> GPAFEFAVAMMKRN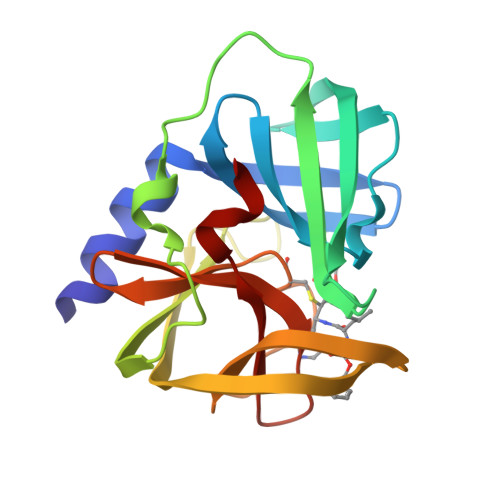SSTVKTEYGEFTMLGIYDRWAVLPRHAKPGPTILMNDQEVGVLDAKELVDKDGTNLELTLLKLNRNEKFRDIRGFLAKEEVEVNEAVLAINTSKFPNMYIPVGQVTEYGFLNLGGTPTKRMLMYNFPTRAGQCGGVLMSTGKVLGIHVGGNGHQGFSAALLKHYFN>MDRQQAERRAAELRELLNRYGYEYYVLDRPSVPDAEYDRLMQELIAIEEQYPELKTSDSPTQRIGGPPLEAFRKVAHRVPMMSLANAFGEGDLRDFDRRVRQEVGEAAYVCELAIDGLAVSVRYEDGYFVQGATRGDGTTGEDITENLKTIRSLPLRLKEPVSLEARGEAFMPKASFLRLNEERKARGEELFANPRNAAAGSLRQLDPKVAASRQLDLFVYGLADAEALGIASHSEA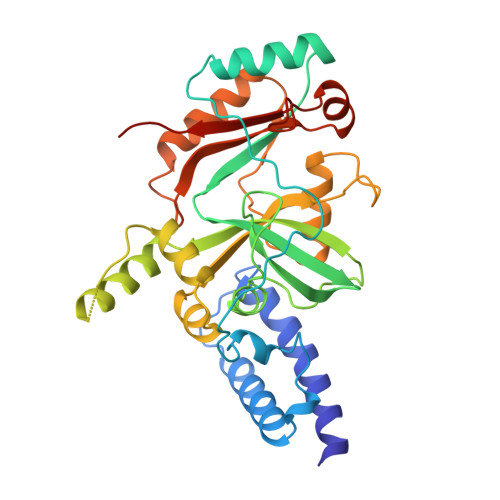LDYLQALGFKVNPERRRCANIDEVIAFVSEWHDKRPQLPYEIDGIVIKVDSFAQQRALGATAKSPRWAIAYKFPAEEVVTT[2x]> DEVAVKMLNSGPGGMMVFDPALVRLKPGDSIKFLPTDKGHNVETIKGMAPDGADYVKTTVGQEAVVKFDKEGVYGFKCAPHYMMGMVALVVVGDKRDNLEAA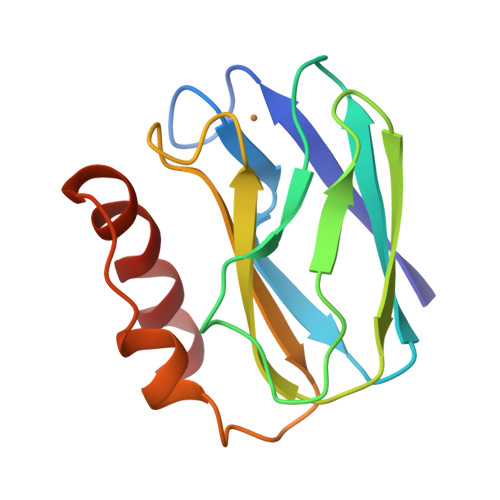KSVQHNKLTQKRLDPLFAQIQ> QKDLADYPVKLKAYEDEQASIKAALAELEKHKNEDGNLTEPSAQNLVYDLEPNANLSLTTDGKFLKASAVDDAFSKSTSKAKYVQKILQLDDLDITNLEQSNDVASSMELYGNFGDKAGWSTTVSNNSQVKWGSVLLERGQSATATYTNLQNSYYNGKKISKIVYKYTVDPKSKFQGQKVWLGIFTDPTLGVFASAYTGQVEKNTSIFIKNEFTFYDEDGKPINFDNALLSVASLNREHNSIEMAKDYSGKFVKISGSSIGEK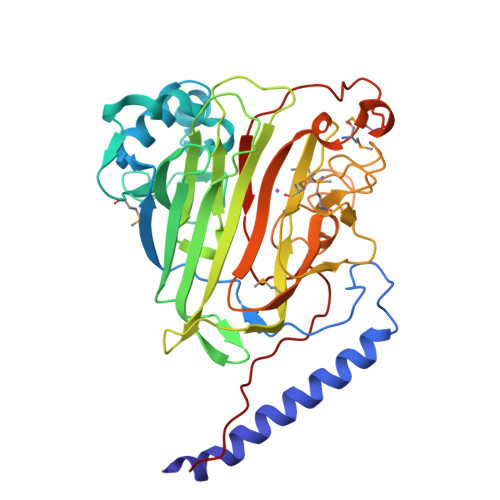NGMIYATDTLNFKQGEGGSRWTMYKNSQAGSGWDSSDAPNSWYGAGAIKMSGPNNHVTVGATSATNVMPVSDMPVVPGKDNTDGKKPNIWYSLNGKIRAVNVPKVTKEKPTPPV> LALKKKSIPQPTNALKSFNWSKLPENKLEGTVWTEIDDTKVFKILDLEDLERTFSAYQRQQDFFVNSNSKQKEADAIDDTLSSKLKVKELSVIDGRRAQNCNILLSRLKLSNDEIKRAILTMDEQEDLPKDMLEQLLKFVPEKSDIDLLEEHKHELDRMAKADRFLFEMSRINHYQQRLQSLYFKKKFAERVAEVKPKVEAIRSGSEEVFRSGALKQLLEVVLAFGNYMNKGQRGNAYGFKISSLNKIADTKSSIDKNITLLHYLITIVENKYPSVLNLNEELRDIPQAAKVNMTELDKEISTLRSGLKAV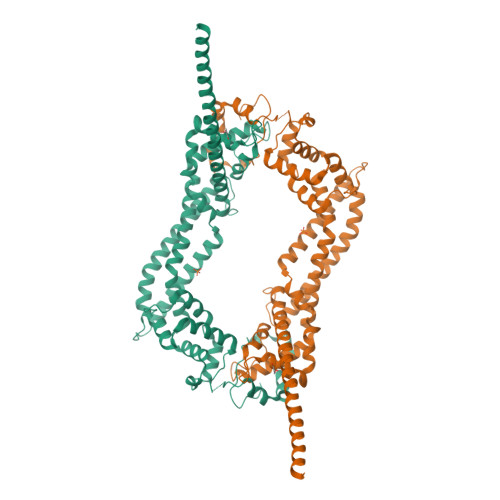ETELEYQKSQPPQPGDKFVSVVSQFITVASFSFSDVEDLLAEAKDLFTKAVKHFGEEAGKIQPDEFFGIFDQFLQAVSEAKQENENMRKKKEEEERRARMEAQLKEQRERERKMRKAKENSEESGEFDDLVSALRSGEVFDKDLSKLKRNRKRITNQMTDSSRERPITKLNF> MPEGADPVAEVKTALAGFLKEVKGFQDDVKTRLQQQEERVTMLQTKTYAGRHALAAAATEEAPHQKAFAAYLRTGDDDGLRGLSLEGKALNSAVAAEGGYLVDPQTSETIRGVLRSTASLRQIASVVNVEATSFDVLVDKTDMGSGWASETAALSETATPQIDRITIPLHELAAMPKASQRLLDDSAFDIETWLANRIADKFARAEAAAFISGDGVDKPTGFLTKTKVANGAWAWGSLGYVATGAAGDFAAVNASDAVVDLVYALGAEYRANASFVMNSKTAGAVRKMKDADGRFLWADSLAAGEPARLMGYPVLIAEDMPDIAANAYAIAFGDFGNGYTIAERPDLRVLRDP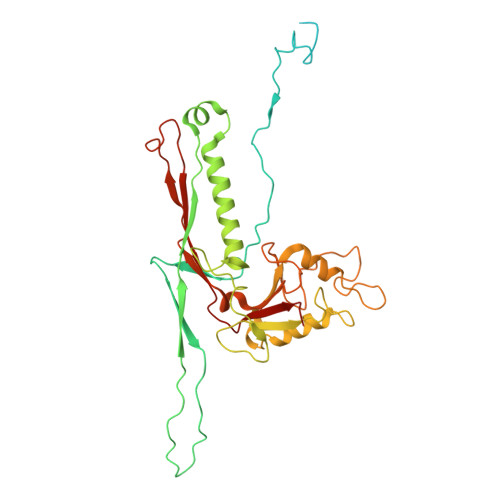FSAKPHVLFYASKRVGGDVSDFAAIKLLKFAAS> MGHHHHHHDIIDVNGITIDKNAFKVTVNGAE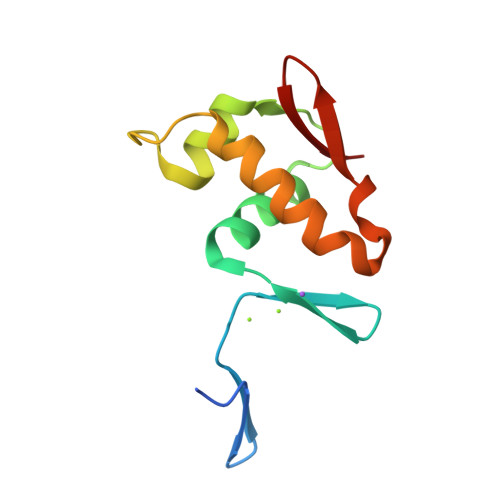IELTKTEYDLLYLLAENKNHVMQREQILNHVWGYNSEVETNVVDVYIRYLRNKLKPYDRDKMIETVRGVGYVIR2-phenoxy-5-(1H-pyrazol-4-yl)benzoic acid | C16 H12 N2 O3 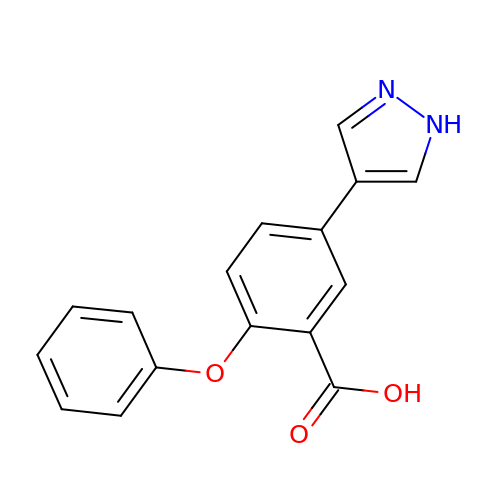| GTIPHUDSAYUQQM-UHFFFAOYSA-N>[2x]MDLLEAKRLLETGRTTPLALLEEALERAKAFQDRNALAYLDEEAARKEALALTEELRRGQVRGPLHGLPLTVKDLFPVKGMPTRAGTKAPLPPLPEEARAVRRLREAGALLFAKTNMHEIALGITGENPWTGPVRNAVDPSRQAGGSSGGSA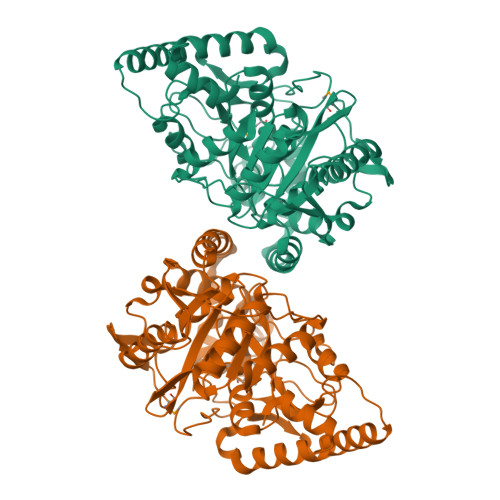VAVALGIGLASLGTDTGGSIRIPAGFNGVVGFKPSYGRVSLEGALPLSRSTDHAGPLTRSVRDAHFLTEILAGESIPLEGVQNPVFGVPLDFLEGRLGVEVRKAFTRLLEDLPALRAEVREVSLPLEGVYEVYTRLVRYEAARIHEKALKEHPEGFSPQVREALLAGLALTEKDYRDAVAEREALRLELVKALRGVDALLLPVQPLPAPPLGTEEVELESGRKGHREAFITLTLPFSLLGVPTLALPFAKVEGMPVGLQVVGAYGEDGKVLALGGWLEARLG> APRQRQSTLVLFPGDLRTNLTDRQLAEEYLYRYGYTRVAEMRGESKSLGPALLLLQKQLSLPETGELDSATLKAMRTPRCGVPDLGRFQTFEGDLKWHHHNITYWIQNYSEDLPRAVIDDAFARAFALWSAVTPLTFTRVYSRDADIVIQFGVAEHGDGYPFDGKDGLLAHAFPPGPGIQGDAHFDDDELWSLGKGVVVPTRFGNADGAACHFPFIFEGRSYSACTTDGRSDGLPWCSTTANYDTDDRFGFCPSERLYTRDGNADGKPCQFPFIFQGQSYSACTTDGRSDGYRWCATTANYDRDKLFGFCPTRADSTVMGGNSAGELCVFPFTFLGKEYSTCTSEGRGDGRLWCATTSNFDSDK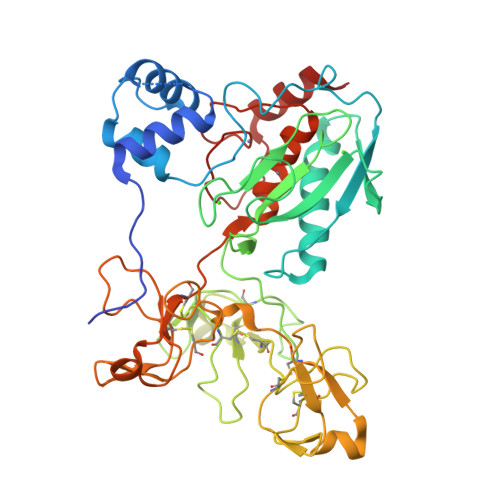KWGFCPDQGYSLFLVAAHEFGHALGLDHSSVPEALMYPMYRFTEGPPLHKDDVNGIRHLYG> GMGSMSTPAASANGGQVLLLPFPAAQGHTNPMLQFGRRLAYHGLRPTLVTTRYVLSTTPPPGDPFRVAAISDGFDDASGMAALPDPGEYLRTLEAHGARTLAELLLSEARAGRPARVLVYDPHLPWARRVARAAGVATAAFLSQPCAVDLIYGEVCARRLALPVTPTDARGLYARGVLGVELGPDDVPPFVAAPELTPAFCEASIEQFAGLEDDDDVLVNSFSDLEPKEAAYMESTWRAKTIGPSLPSFYLDDGRLRSNTAYGFNLFRSTVPCMEWLDKQPPRSVVLVSYGTVSTFDVAKLEELGNGLCNSGKPFLWVVRSNEEHKLSVQLRKKCEKRGLIVPFCPQLEVLAHKATGCFLSHCGWNSTLEAIVNGVPLVAMPHWADQPTIS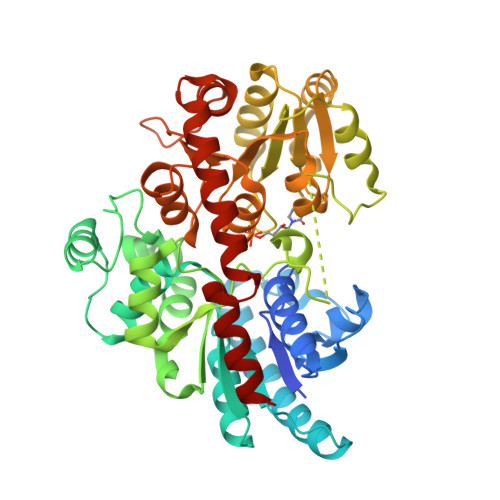KYVESLWGMGVRVQLDKSGILQREEVERCIREVMDGDRKEDYRRNATRLMKKAKESMQEGGSSDKNIAEFAAKYSN>GAASDEYDYLFKVVLIGDSGVGKSN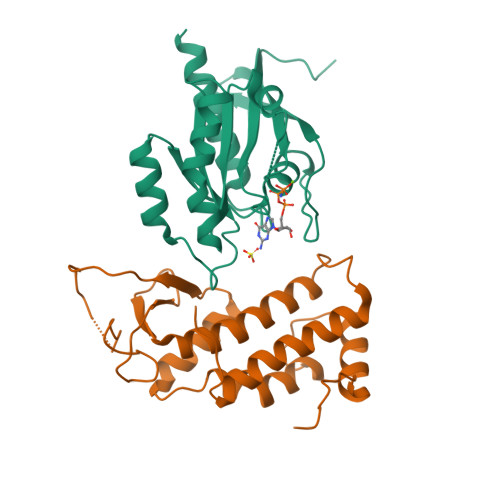LLSRFTRNEFNLESKSTIGVEFATRSIQVDGKTIKAQIWDTAGLERYRAITSAYYRGAVGALLVYDIAKHLTYENVERWLKELRDHADSNIVIMLVGNKSDLRHLRAVPTDEARAFAEKNGLSFIETSALDSTNVEAAFQTILTEIYRIVSQKQMSDRRE[2x];>[2x]GAASNKSTSSAMSGSHQDLSVIQPIVKDCKEADLSLYNEFRLWKDEPTMDRTCPFLDKIYQEDIFPCLTFSKSELASAVLEAVENNTLSIEPVGLQPIRFVKASAVECGGPKKCALTGQSKSCKHRIKLGDSSNYYYISPFCRYRITSVCNFFTYIRYIQQGLVKQQDVDQMFWEVMQLRKEMSLAKLGYFKEEL>MAPKAVLVGLPGSGKSTIGRRLAKALGVGLLDTDVAIEQRTGRSIADIFATDGEQEFRRIEEDVVRAALADHDGVLSLGGGAVTSPGVRAALAGHTVVYLEISAAEGVRRTGGNTVRPLLAGPDRAEKYRA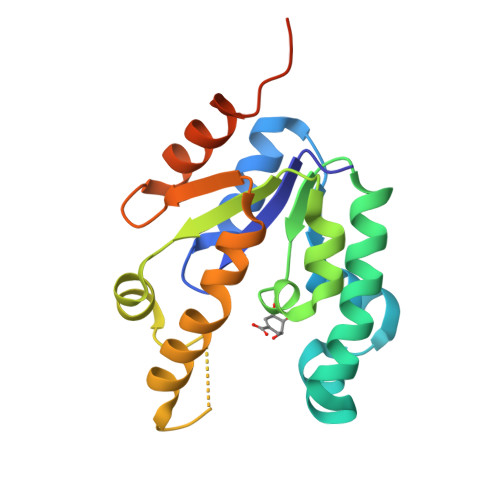LMAKRAPLYRRVATMRVDTNRRNPGAVVRHILSRLQVPSPSEAATLEHHHHHH[2x]>[6x]MGGEVEEPEPQMVLSPLTSAAIFL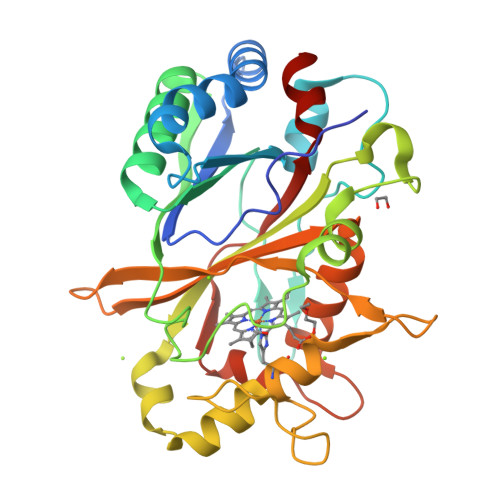VVTIDSGGEDTVRDLLSDVASLERAVGFRAQPDGRLSCVTGIGSEAWDRLFSGARPAGLHPFRELDGPVHRAVATPGDLLFHIRASRLDLCFALATEIMGRLRGAVTPQDEVHGFKYFDERDMLGFVDGTENPTGAAARRAVLVGAEDPAFAGGSYAVVQKYLHDIDAWEGLSVEAQERVIGRRKMTDVELSDDVKPADSHVALTSVTGPDGSDLEILRDNMPFGSVGREEFGTYFIGYARTPEVTETMLERMFLGTASAPHDRILDFSTAVTGSLFFTPAADFLEDLSARP tert-butyl N-[3-(2-hydroxyethylcarbamoyl)-5-phenyl-thiophen-2-yl]carbamate | C18 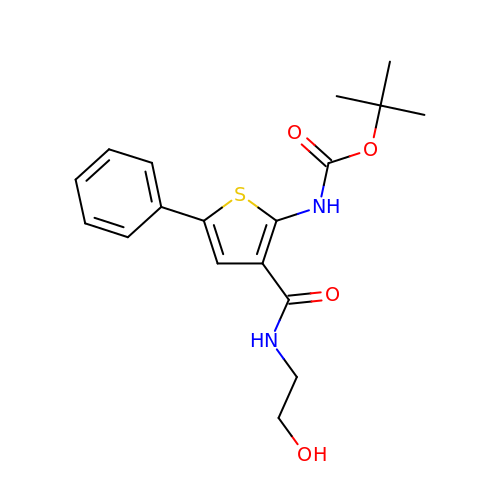H22 N2 O4 S | IBSJNIANIOEIGQ-UHFFFAOYSA-N> MSSKEQKTPEGQAPEEIIMDQHEEIEAVEPEASAEQVDPRDEKVANLEAQ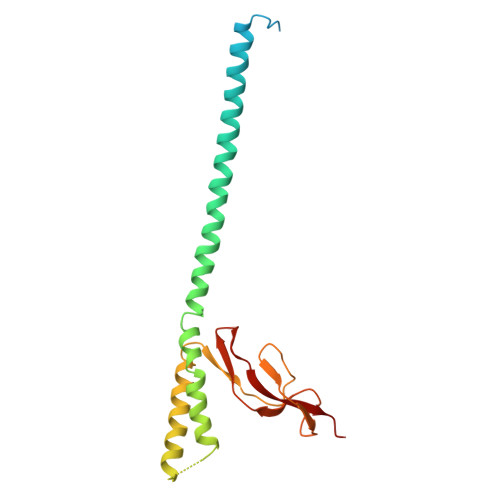LAEAQTRERDGILRVKAEMENLRRRTELDIEKAHKFALEKFINELLPVIDSLDRALEVADKANPDMSAMVEDIELTLKSMLDVVRKFGVEVIAETNVPLDPNVHQAIAMVESDDVAPGNVLGIMQKGYTLNGRTIRAAMVTVAKAKA> MSLDCRERIEKDLELLEKNLMEMKSIKLSDDEEAVVERALNYRDDSVYYLEKGDHITSFGCITYAHGLLDSLRMLHR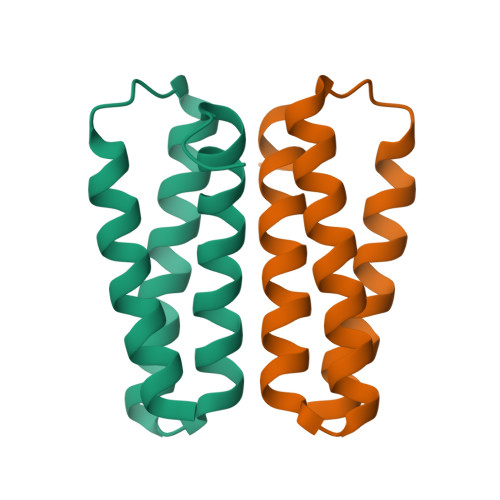IIEGHHHHHH heptyl alpha-D-mannopyranoside | C13 H26 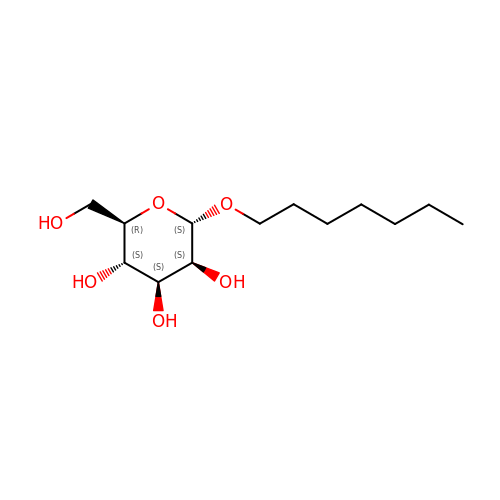O6 | NIDYWHLDTIVRJT-BNDIWNMDSA-N>AMNAFGDMTSEEFRQVMNGFQNRKPRKGKVFQEPLFYEAPRSVDWREKGYVTPVKNQGQCGSCWAFSATGALEGQMFRKTGRLISLSEQNLVDCSGPQGNEGCNGGLMDYAFQYVQDNGGLDSEESYPYEATEESCKYNPKYSVANDAGFVDIPKQEKALMKAVATVGPISVAIDAGHESFLFYKEGIYFEPDCSSEDM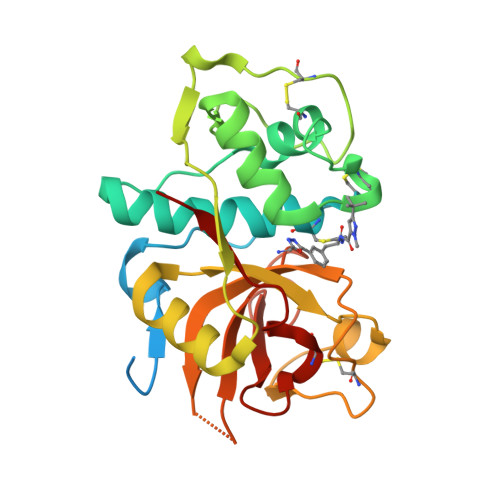DHGVLVVGYGFESTESDNNKYWLVKNSWGEEWGMGGYVKMAKDRRNHCGIASAASYPTV[4x]> DCPSGWSSYEGNCYKFFQQKMNWADAERFCSEQAKGGHLVSIKIYSKEKDFVGDLVTKNIQSSDLYAWIGLRVENKEKQCSSEWSDGSSVSYENVVERTVKKCFALEKDLGFVLWINLYCAQKNPFVC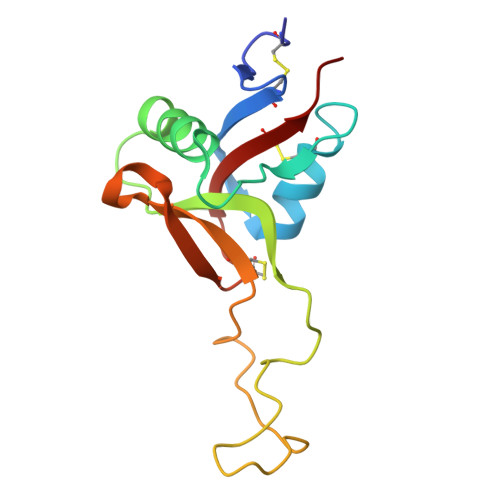KSPPP>XGLLEEIAQLLEEIAKLLKKIAWLLKKIAQGX[6x]

Here we describe efficient routes starting from validated parallel and antiparallel peptide assemblies to design two families of α-helical barrel proteins with central channels that bind small molecules. Computational designs are seeded by the sequences and structures of defined de novo oligomeric barrel-forming peptides, and adjacent helices are connected by loop building. For targets with antiparallel helices, short loops are sufficient. However, targets with parallel helices require longer connectors; namely, an outer layer of helix–turn–helix–turn–helix motifs that are packed onto the barrels.

We solved high-resolution X-ray crystal structures of three peptides using ab initio phasing. We named this peptide apCC-Hex-LLIA, and systematically as apCC-Hex. Using the experimental apCC-Hex structure as a seed, we designed short loop sequences computationally to connect adjacent helices to generate an up-down α-meander structure. For the antiparallel α-helical barrel proteins, the seeds, models and experimental structures for sc-apCC-6-LLIA and sc-apCC-8 are very similar.>[2x]GAMAPHFKEELRNLNVRYQSNATLVCKVTGHPKPIVKWYRQGKEIIADGLKYRIQEFKGGYHQLIIASVTDDDATVYQVRATNQGGSVSGTASLEVEVPAKIHLPKTLEGMGAVHALR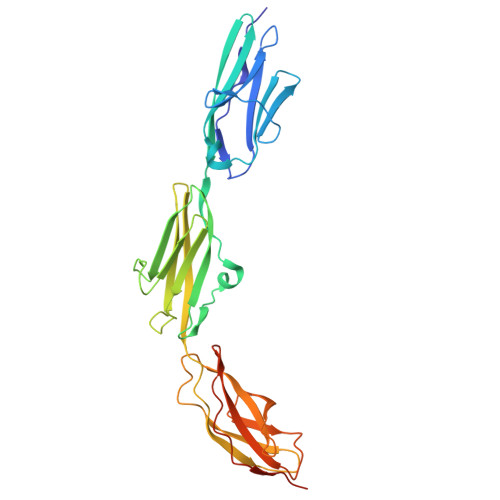GEVVSIKIPFSGKPDPVITWQKGQDLIDNNGHYQVIVTRSFTSLVFPNGVERKDAGFYVVCAKNRFGIDQKTVELDVADVPDPPRGVKVSDVSRDSVNLTWTEPASDGGSKITNYIVEKCATTAERWLRVGQARETRYTVINLFGKTSYQFRVIAENKFGLSKPSEPSEPTITKEDKTRAMNYDEEV>SIEKIWAREILDSRGNPTVEVDLYTAKGLFRAAVPSGASTGIYEALELRDGDKQRYLGKGVLKAVDHINSTIAPALISSGLSVVEQEKLDNLMLELDGTENKSKFGANAILGVSLAVCKAGAAERELPLYRHIAQLAGNSDLILPVPAFNVINGGSHAGNKLAMQEFMILPVGAESFRDAMRLGAEVYHTLKGVIKDKYGKDATNVGDEGGFAPNILENSEALELVKEAIDKAGYTEKIVIGMDVAASEFYRDGKYDLDFKSPTDPSRYITGDQLGALYQDFVRDYPVVSIEDPFDQDDWAAWSKFTANVGIQIVGDDLTVTNPKRIERAVEEKACNCLLLKVNQIGSVTEAIQACKLAQENGWGVMVSHRSGETEDTFIADLVVGLCTGQIKTGAPCRSERLAKYNQLMRIEEELGDEARF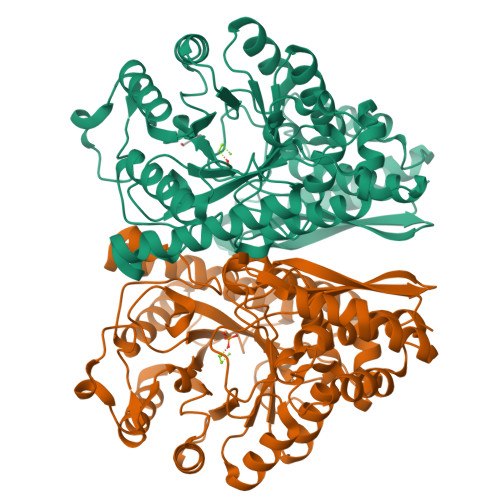AGHNFRNPSVLHHHHHH[2x]> CATTAGCGTCAGACGATAAATTTAGCCGGAACTAAAACACTCTTGTATCATCGCCTTGTAGCG;> ATTAAAGATCGGCACGGAGATATCTTTGACCCCCACTAAAACCGCTTTT;> AAGGGCGACATTCAATAAGTTTACCAGAATGAAATTTTACAG;> TTTTTTTTTTTGGTTTACCAGCGCCACAATAGAAAGCAGA;> TTTTTTTTTTTAGTCAGAAGCAACTCCAACAGGTTTTTTTTTTT;> AAGCGGAGGAGAAGGAACCCTAAATCACCATCAATATGATTTTTTTTTTT;> TTGCATCAAATCAGTAAATATTCATTGACCAGAGGGGGTAATAGTAAAA;> CAAACGTGACTCCTCGCTAATTGAACAAAGTCAGACTCCTCA;> TATTTTGTCACAATAAGACAAGGAACCAGAGCCACCACCGTTTTTTTTTT;> AATTCGAGCTTCAAAGCGAACTCCTTTTCTGTAGCTCAACATGTTTTAA;> TGATAGACGGTTTTTCGCCCTTTGACGTTGGAGTCCACGTTCTTTAATAGTGGACTCTTGTTCCAAACTGGAACAACACTCAACCCTATCTCGGGCTATTCTTTTGATTTATAAGGGATTTTGCCGATTTCGGAACCACCATCAAACAGGATTTTCGCCTGCTGGGGCAAACCAGCGTGGACCGCTTGCTGCAACTCTCTCAGGGCCAGGCGGTGAAGGGCAATCAGCTGTTGCCCGTCTCACTGGTGAAAAGAAAAACCACCCTGGCGCCCAATACGCAAACCGCCTCTCCCCGCGCGTTGGCCGATTCATTAATGCAGCTGGCACGACAGGTTTCCCGACTGGAAAGCGGGCAGTGAGCGCAACGCAATTAATGTGAGTTAGCTCACTCATTAGGCACCCCAGGCTTTACACTTTATGCTTCCGGCTCGTATGTTGTGTGGAATTGTGAGCGGATAACAATTTCACACAGGAAACAGCTATGACCATGATTACGAATTCGAGCTCGGTACCCGGGGATCCTCAACTGTGAGGAGGCTCACGGACGCGAAGAACAGGCACGCGTGCTGGCAGAAACCCCCGGTATGACCGTGAAAACGGCCCGCCGCATTCTGGCCGCAGCACCACAGAGTGCACAGGCGCGCAGTGACACTGCGCTGGATCGTCTGATGCAGGGGGCACCGGCACCGCTGGCTGCAGGTAACCCGGCATCTGATGCCGTTAACGATTTGCTGAACACACCAGTGTAAGGGATGTTTATGACGAGCAAAGAAACCTTTACCCATTACCAGCCGCAGGGCAACAGTGACCCGGCTCATACCGCAACCGCGCCCGGCGGATTGAGTGCGAAAGCGCCTGCAATGACCCCGCTGATGCTGGACACCTCCAGCCGTAAGCTGGTTGCGTGGGATGGCACCACCGACGGTGCTGCCGTTGGCATTCTTGCGGTTGCTGCTGACCAGACCAGCACCACGCTGACGTTCTACAAGTCCGGCACGTTCCGTTATGAGGATGTGCTCTGGCCGGAGGCTGCCAGCGACGAGACGAAAAAACGGACCGCGTTTGCCGGAACGGCAATCAGCATCGTTTAACTTTACCCTTCATCACTAAAGGCCGCCTGTGCGGCTTTTTTTACGGGATTTTTTTATGTCGATGTACACAACCGCCCAACTGCTGGCGGCAAATGAGCAGAAATTTAAGTTTGATCCGCTGTTTCTGCGTCTCTTTTTCCGTGAGAGCTATCCCTTCACCACGGAGAAAGTCTATCTCTCACAAATTCCGGGACTGGTAAACATGGCGCTGTACGTTTCGCCGATTGTTTCCGGTGAGGTTATCCGTTCCCGTGGCGGCTCCACCTCTGAAAGCTTGGCACTGGCCGTCGTTTTACAACGTCGTGACTGGGAAAACCCTGGCGTTACCCAACTTAATCGCCTTGCAGCACATCCCCCTTTCGCCAGCTGGCGTAATAGCGAAGAGGCCCGCACCGATCGCCCTTCCCAACAGTTGCGCAGCCTGAATGGCGAATGGCGCTTTGCCTGGTTTCCGGCACCAGAAGCGGTGCCGGAAAGCTGGCTGGAGTGCGATCTTCCTGAGGCCGATACTGTCGTCGTCCCCTCAAACTGGCAGATGCACGGTTACGATGCGCCCATCTACACCAACGTGACCTATCCCATTACGGTCAATCCGCCGTTTGTTCCCACGGAGAATCCGACGGGTTGTTACTCGCTCACATTTAATGTTGATGAAAGCTGGCTACAGGAAGGCCAGACGCGAATTATTTTTGATGGCGTTCCTATTGGTTAAAAAATGAGCTGATTTAACAAAAATTTAATGCGAATTTTAACAAAATATTAACGTTTACAATTTAAATATTTGCTTATACAATCTTCCTGTTTTTGGGGCTTTTCTGATTATCAACCGGGGTACATATGATTGACATGCTAGTTTTACGATTACCGTTCATCGATTCTCTTGTTTGCTCCAGACTCTCAGGCAATGACCTGATAGCCTTTGTAGATCTCTCAAAAATAGCTACCCTCTCCGGCATTAATTTATCAGCTAGAACGGTTGAATATCATATTGATGGTGATTTGACTGTCTCCGGCCTTTCTCACCCTTTTGAATCTTTACCTACACATTACTCAGGCATTGCATTTAAAATATATGAGGGTTCTAAAAATTTTTATCCTTGCGTTGAAATAAAGGCTTCTCCCGCAAAAGTATTACAGGGTCATAATGTTTTTGGTACAACCGATTTAGCTTTATGCTCTGAGGCTTTATTGCTTAATTTTGCTAATTCTTTGCCTTGCCTGTATGATTTATTGGATGTTAATGCTACTACTATTAGTAGAATTGATGCCACCTTTTCAGCTCGCGCCCCAAATGAAAATATAGCTAAACAGGTTATTGACCATTTGCGAAATGTATCTAATGGTCAAACTAAATCTACTCGTTCGCAGAATTGGGAATCAACTGTTATATGGAATGAAACTTCCAGACACCGTACTTTAGTTGCATATTTAAAACATGTTGAGCTACAGCATTATATTCAGCAATTAAGCTCTAAGCCATCCGCAAAAATGACCTCTTATCAAAAGGAGCAATTAAAGGTACTCTCTAATCCTGACCTGTTGGAGTTTGCTTCCGGTCTGGTTCGCTTTGAAGCTCGAATTAAAACGCGATATTTGAAGTCTTTCGGGCTTCCTCTTAATCTTTTTGATGCAATCCGCTTTGCTTCTGACTATAATAGTCAGGGTAAAGACCTGATTTTTGATTTATGGTCATTCTCGTTTTCTGAACTGTTTAAAGCATTTGAGGGGGATTCAATGAATATTTATGACGATTCCGCAGTATTGGACGCTATCCAGTCTAAACATTTTACTATTACCCCCTCTGGCAAAACTTCTTTTGCAAAAGCCTCTCGCTATTTTGGTTTTTATCGTCGTCTGGTAAACGAGGGTTATGATAGTGTTGCTCTTACTATGCCTCGTAATTCCTTTTGGCGTTATGTATCTGCATTAGTTGAATGTGGTATTCCTAAATCTCAACTGATGAATCTTTCTACCTGTAATAATGTTGTTCCGTTAGTTCGTTTTATTAACGTAGATTTTTCTTCCCAACGTCCTGACTGGTATAATGAGCCAGTTCTTAAAATCGCATAAGGTAATTCACAATGATTAAAGTTGAAATTAAACCATCTCAAGCCCAATTTACTACTCGTTCTGGTGTTTCTCGTCAGGGCAAGCCTTATTCACTGAATGAGCAGCTTTGTTACGTTGATTTGGGTAATGAATATCCGGTTCTTGTCAAGATTACTCTTGATGAAGGTCAGCCAGCCTATGCGCCTGGTCTGTACACCGTTCATCTGTCCTCTTTCAAAGTTGGTCAGTTCGGTTCCCTTATGATTGACCGTCTGCGCCTCGTTCCGGCTAAGTAACATGGAGCAGGTCGCGGATTTCGACACAATTTATCAGGCGATGATACAAATCTCCGTTGTACTTTGTTTCGCGCTTGGTATAATCGCTGGGGGTCAAAGATGAGTGTTTTAGTGTATTCTTTTGCCTCTTTCGTTTTAGGTTGGTGCCTTCGTAGTGGCATTACGTATTTTACCCGTTTAATGGAAACTTCCTCATGAAAAAGTCTTTAGTCCTCAAAGCCTCTGTAGCCGTTGCTACCCTCGTTCCGATGCTGTCTTTCGCTGCTGAGGGTGACGATCCCGCAAAAGCGGCCTTTAACTCCCTGCAAGCCTCAGCGACCGAATATATCGGTTATGCGTGGGCGATGGTTGTTGTCATTGTCGGCGCAACTATCGGTATCAAGCTGTTTAAGAAATTCACCTCGAAAGCAAGCTGATAAACCGATACAATTAAAGGCTCCTTTTGGAGCCTTTTTTTTGGAGATTTTCAACGTGAAAAAATTATTATTCGCAATTCCTTTAGTTGTTCCTTTCTATTCTCACTCCGCTGAAACTGTTGAAAGTTGTTTAGCAAAATCCCATACAGAAAATTCATTTACTAACGTCTGGAAAGACGACAAAACTTTAGATCGTTACGCTAACTATGAGGGCTGTCTGTGGAATGCTACAGGCGTTGTAGTTTGTACTGGTGACGAAACTCAGTGTTACGGTACATGGGTTCCTATTGGGCTTGCTATCCCTGAAAATGAGGGTGGTGGCTCTGAGGGTGGCGGTTCTGAGGGTGGCGGTTCTGAGGGTGGCGGTACTAAACCTCCTGAGTACGGTGATACACCTATTCCGGGCTATACTTATATCAACCCTCTCGACGGCACTTATCCGCCTGGTACTGAGCAAAACCCCGCTAATCCTAATCCTTCTCTTGAGGAGTCTCAGCCTCTTAATACTTTCATGTTTCAGAATAATAGGTTCCGAAATAGGCAGGGGGCATTAACTGTTTATACGGGCACTGTTACTCAAGGCACTGACCCCGTTAAAACTTATTACCAGTACACTCCTGTATCATCAAAAGCCATGTATGACGCTTACTGGAACGGTAAATTCAGAGACTGCGCTTTCCATTCTGGCTTTAATGAGGATTTATTTGTTTGTGAATATCAAGGCCAATCGTCTGACCTGCCTCAACCTCCTGTCAATGCTGGCGGCGGCTCTGGTGGTGGTTCTGGTGGCGGCTCTGAGGGTGGTGGCTCTGAGGGTGGCGGTTCTGAGGGTGGCGGCTCTGAGGGAGGCGGTTCCGGTGGTGGCTCTGGTTCCGGTGATTTTGATTATGAAAAGATGGCAAACGCTAATAAGGGGGCTATGACCGAAAATGCCGATGAAAACGCGCTACAGTCTGACGCTAAAGGCAAACTTGATTCTGTCGCTACTGATTACGGTGCTGCTATCGATGGTTTCATTGGTGACGTTTCCGGCCTTGCTAATGGTAATGGTGCTACTGGTGATTTTGCTGGCTCTAATTCCCAAATGGCTCAAGTCGGTGACGGTGATAATTCACCTTTAATGAATAATTTCCGTCAATATTTACCTTCCCTCCCTCAATCGGTTGAATGTCGCCCTTTTGTCTTTGGCGCTGGTAAACCATATGAATTTTCTATTGATTGTGACAAAATAAACTTATTCCGTGGTGTCTTTGCGTTTCTTTTATATGTTGCCACCTTTATGTATGTATTTTCTACGTTTGCTAACATACTGCGTAATAAGGAGTCTTAATCATGCCAGTTCTTTTGGGTATTCCGTTATTATTGCGTTTCCTCGGTTTCCTTCTGGTAACTTTGTTCGGCTATCTGCTTACTTTTCTTAAAAAGGGCTTCGGTAAGATAGCTATTGCTATTTCATTGTTTCTTGCTCTTATTATTGGGCTTAACTCAATTCTTGTGGGTTATCTCTCTGATATTAGCGCTCAATTACCCTCTGACTTTGTTCAGGGTGTTCAGTTAATTCTCCCGTCTAATGCGCTTCCCTGTTTTTATGTTATTCTCTCTGTAAAGGCTGCTATTTTCATTTTTGACGTTAAACAAAAAATCGTTTCTTATTTGGATTGGGATAAATAATATGGCTGTTTATTTTGTAACTGGCAAATTAGGCTCTGGAAAGACGCTCGTTAGCGTTGGTAAGATTCAGGATAAAATTGTAGCTGGGTGCAAAATAGCAACTAATCTTGATTTAAGGCTTCAAAACCTCCCGCAAGTCGGGAGGTTCGCTAAAACGCCTCGCGTTCTTAGAATACCGGATAAGCCTTCTATATCTGATTTGCTTGCTATTGGGCGCGGTAATGATTCCTACGATGAAAATAAAAACGGCTTGCTTGTTCTCGATGAGTGCGGTACTTGGTTTAATACCCGTTCTTGGAATGATAAGGAAAGACAGCCGATTATTGATTGGTTTCTACATGCTCGTAAATTAGGATGGGATATTATTTTTCTTGTTCAGGACTTATCTATTGTTGATAAACAGGCGCGTTCTGCATTAGCTGAACATGTTGTTTATTGTCGTCGTCTGGACAGAATTACTTTACCTTTTGTCGGTACTTTATATTCTCTTATTACTGGCTCGAAAATGCCTCTGCCTAAATTACATGTTGGCGTTGTTAAATATGGCGATTCTCAATTAAGCCCTACTGTTGAGCGTTGGCTTTATACTGGTAAGAATTTGTATAACGCATATGATACTAAACAGGCTTTTTCTAGTAATTATGATTCCGGTGTTTATTCTTATTTAACGCCTTATTTATCACACGGTCGGTATTTCAAACCATTAAATTTAGGTCAGAAGATGAAATTAACTAAAATATATTTGAAAAAGTTTTCTCGCGTTCTTTGTCTTGCGATTGGATTTGCATCAGCATTTACATATAGTTATATAACCCAACCTAAGCCGGAGGTTAAAAAGGTAGTCTCTCAGACCTATGATTTTGATAAATTCACTATTGACTCTTCTCAGCGTCTTAATCTAAGCTATCGCTATGTTTTCAAGGATTCTAAGGGAAAATTAATTAATAGCGACGATTTACAGAAGCAAGGTTATTCACTCACATATATTGATTTATGTACTGTTTCCATTAAAAAAGGTAATTCAAATGAAATTGTTAAATGTAATTAATTTTGTTTTCTTGATGTTTGTTTCATCATCTTCTTTTGCTCAGGTAATTGAAATGAATAATTCGCCTCTGCGCGATTTTGTAACTTGGTATTCAAAGCAATCAGGCGAATCCGTTATTGTTTCTCCCGATGTAAAAGGTACTGTTACTGTATATTCATCTGACGTTAAACCTGAAAATCTACGCAATTTCTTTATTTCTGTTTTACGTGCAAATAATTTTGATATGGTAGGTTCTAACCCTTCCATTATTCAGAAGTATAATCCAAACAATCAGGATTATATTGATGAATTGCCATCATCTGATAATCAGGAATATGATGATAATTCCGCTCCTTCTGGTGGTTTCTTTGTTCCGCAAAATGATAATGTTACTCAAACTTTTAAAATTAATAACGTTCGGGCAAAGGATTTAATACGAGTTGTCGAATTGTTTGTAAAGTCTAATACTTCTAAATCCTCAAATGTATTATCTATTGACGGCTCTAATCTATTAGTTGTTAGTGCTCCTAAAGATATTTTAGATAACCTTCCTCAATTCCTTTCAACTGTTGATTTGCCAACTGACCAGATATTGATTGAGGGTTTGATATTTGAGGTTCAGCAAGGTGATGCTTTAGATTTTTCATTTGCTGCTGGCTCTCAGCGTGGCACTGTTGCAGGCGGTGTTAATACTGACCGCCTCACCTCTGTTTTATCTTCTGCTGGTGGTTCGTTCGGTATTTTTAATGGCGATGTTTTAGGGCTATCAGTTCGCGCATTAAAGACTAATAGCCATTCAAAAATATTGTCTGTGCCACGTATTCTTACGCTTTCAGGTCAGAAGGGTTCTATCTCTGTTGGCCAGAATGTCCCTTTTATTACTGGTCGTGTGACTGGTGAATCTGCCAATGTAAATAATCCATTTCAGACGATTGAGCGTCAAAATGTAGGTATTTCCATGAGCGTTTTTCCTGTTGCAATGGCTGGCGGTAATATTGTTCTGGATATTACCAGCAAGGCCGATAGTTTGAGTTCTTCTACTCAGGCAAGTGATGTTATTACTAATCAAAGAAGTATTGCTACAACGGTTAATTTGCGTGATGGACAGACTCTTTTACTCGGTGGCCTCACTGATTATAAAAACACTTCTCAGGATTCTGGCGTACCGTTCCTGTCTAAAATCCCTTTAATCGGCCTCCTGTTTAGCTCCCGCTCTGATTCTAACGAGGAAAGCACGTTATACGTGCTCGTCAAAGCAACCATAGTACGCGCCCTGTAGCGGCGCATTAAGCGCGGCGGGTGTGGTGGTTACGCGCAGCGTGACCGCTACACTTGCCAGCGCCCTAGCGCCCGCTCCTTTCGCTTTCTTCCCTTCCTTTCTCGCCACGTTCGCCGGCTTTCCCCGTCAAGCTCTAAATCGGGGGCTCCCTTTAGGGTTCCGATTTAGTGCTTTACGGCACCTCGACCCCAAAAAACTTGATTTGGGTGATGGTTCACGTAGTGGGCCATCGCCC;> TTTTTTTTTTACTAAAGACTTTTTCATACAGAGGGAGCCT;> TTTTTTTTTTACAGACCAGGCGAGCTGCTCATTCTTTTTTTTTT;> CATAGGCTGGCTGATTTGAAAGAGGACAGATGAACGGTGTTTTTTTTTTT;> CCTTCATTTACCCAAACACCAAATTTCACCAGTCAGGACGTTGGGAA;> GGCTTGCGACAACATAAACAAGTCTTTCCAGACGTTAGTAAAGTATGGG;> CTCAGCAGAATTTCAACAACTCAGACAGCCCTCATAGTTAGCTGAGAAT;> AGGGTAGCAACGGCTGAGGAAGTTTCCATTAAACGCGGAACGTTATCAG;> GTTGCGCCGACAATAGGGAGTCAGAGCCCGTTTTCGTGAATTATCACAA;> ACCGATAAGCGGAGGTAACGATCTAAAGTTTTGTCCTTTCAA;> TTAAACAGCTTGATGCGGGATAGCCGCCTCATAGCGACGGAATTAGAGCCAGCA;> TTTTTTTTTTGCTCCAAAAGCTTTGAGGTTTTTTTTTT;> TTTTTTTTTTAGTGAATAAGGCGAATTACCTTATTTTTTTTTTT;> TAATAATTACAACGTTTCAGGGATAGCATACCGCC;> AATCTCCAGTTTCGTAGGAACCCATGTACCTTTTTTTTTT;> ACTTTAATCATTGTTTGCCCTAATTACGCGTTTACGAAGCAA;> TGAATGGGCTTGAGATGGTTTGAACGAGCAGATAC;> CCTGTAGCATTCCAAAAGGAAGGGTCAGAAAGCGCCGAGGAAAAAGACA;> TCACCAGTACAAACTTTTTCATACTGGTCCGTTCCACAAAGT;> TTTTTTTTTTGTAACACTGAAAAAAAAGTTTTTTTTTT;> AGCGCGAAACAAAGTACAATTTTCGGACCAGAAAAATAAATATAAAC;> ACCTGCTCCCAATCATACCGATATATTCGGCAGGAGG;> GAAAAATCTACGTTCAACTTATAATGGATAAGAAATAGTATAAAGCTAAATCGG;> TTTTTTTTTTCCGTACTCAGGAGGTTTAGAGCCCAA;> TTTTTTTTTTGCGATTTTAAGAACTGGCTTAACGGA;> ACCCTCAGAGCCACCACACCCTCTGCCGTCAACATAAAAGAGCA;> TTTTTTTTTTTAGAAAGATGTAAGAGCATTTTTTTTTT;> TTGAGATTTAGGAACAAAAGGGACGAGAAATCAACGTAACAA;> GGGTTTTGCTCAGTATTAGACAATTGAGTTTTATTCAAGAAATCATTTG;> GAGAGGGTTTAACGTTGCGAACTTGCTTTCGAGGTGCGAAAG;> AAGTATAAGCAGCCAGCAATATATTAAAACCAATCAAACAAA;> GCCCGGAAGGAGTGCGTTGAATTAATTGTATCGGT;> AGGCATATCATCAGACAACATTATTACAGGTTTTTTTTTT;> TCTGAAACATGATGTAGTAAAGAACCGGATATTCACAAGAGT;> CTATTATGGCAGGTCAATATCGCGTTTTTTTGCGGATGGCGT;> TCGGAACATTTTGCACCATCGCCCACGCATAACAATTTTTCT;> GCCCCCTTGATATTTGATTAAAGAAAATCAGACGAAGTATCA;> GTGCCCGTCCTCATGAATACCGGCAACAAAAAGGTATTCTTA;> TTTTTTTTTTTTTTGATGATACATAGGTGTATCATTTTTTTTTT;> TTTTTTTTTTACACTATCAACTGGATAGTTTTTTTTTT;> CAGACGACGATAAAATAACGCTACCACATTAATAAAACGAACCATTATA;> AACCAAAATAGCGACAAAAGAAATCTTGAAGGGAACCGAACTGACCAAC;> TAAAGCCCCCTCAGCGTCACCACGAAGGCACCAACGCGATTATACCA;> GAATTTAAATAAGTTTGATATACCCTCAGAACCGCCCCTCAT;> AGTTTTGATCCCCCTGACCATAAATCAAAAAAAGATTAAGAG;> GCATTGATCGCTGAGAGGCGCAGACGGTATGTTACTGTGTCGAAATCCGCG;> GCCGCCATTGGCCTGCCTATTAGAGAAGGATTAGGAACACCCATCAGAG;> GCCACCAAGAATGGTGCCTTGGGATAAGAGAACCGCC;> CCTCAGATTGCCATGAGGGAGGGAAGGTGAAACGCACGCAAT;> TTTTTTTTTTGAACCGCCTCCCGTCATACATGGCTTTTTTTTTT;> TTTTTTTTTTCGTCCAATACTGCGGATGTTTAGTAACCCT;> ATCGTCAGTCTTTACCCTGACTATTATTTTTTTTTT;> GATTAAGAATCATATCGCCATATTTAACAACGCTTTTTTTTTT;> AGGTCATTGCCTGAAGAGGGTAACCAGGCAGCTGGTGGGTAACGCCAGG;> TTTTTTTTTTTACCTGAGCGAAGAGTCATTTTTTTTTT;> TTTTTTTTTTTAATCGTAAAACATTTTGTTAAAATTTTTTTTTT;> TATGTACATTTAAACTCATTTTTTAACCGGCCTTC;> ACATCGGTTTTTTAAGATAAGTTCTGTCACATACA;> CTGATTGTTTGCACGTAAAACTCCCGACAAGCCGTTTAAGCCAATAACG;> TTACAAAGAACCTAAGATGATGGCAATTCCAGAAGTTAAAAGTTTGAGT;> ATCGCGCCAGTTGGCACCTTGAGAAAGCAACAGGAGGCCGAT;> AATTATTTTCTGAAATAATCCTGATTGTTTTTTTTT;> ACTGGCACACAAACCCACCACTAAAGGCGAAAGAGGCAAAAGAATACAC;> CAAAAGACCACAAGGGGAGAATTAACTGATTAGCGAGTTAATCAGTTTC;> AGGAAACAGTCTCTCCGCCACACAGCATGGTAAAATACGTAATGCCACT;> TTTTTTTTTTAAGAAAAGTAAATTCATATTTTTTTTTT;> TTTTTTTTTTCAGGATTAGAGAATATGCAACTAATTTTTTTTTT;> GTACCTTCAATAAAAAGCAATCAAGAGATAGCTGATAAATTA;> CAATAATAAACAGGGAAGCGCACCAGGCAGTAACAAGAAAGG;> TACCGAATCAAAAAATAAGAAACGATTTTTTTTTTTTTTT;> GGTTAGAGCTTAATTGCTGAAAAAAGTATTAAGAGGCTGAGA;> TTTTTTTTTTTGTTTAACGGCCCTTTTTTTTTTTTTTT;> ATTCTGCGAACGCGCGAGCAGCAAATCCCGGTT;> TTTTTTTTTTTACAATTTTATCCTGAATCAATCCAATGAAAAT;> TTTTTTTTTTAGTACGGTGTCTGGAAGTTGACCATTTAGCTAT;> TGCCAGTTACAAAATATTTCCAGAGGTTTTAAAATTACTTTGAAAAAGGAA;> ATATTATTTATCCCTTACCAAAGATTAGAGGGTTA;> AAATCACCAGTAGCACCATTATACAAAAAGTAATCCTGAA;> GCAGCACCGTCAGAAAGAAAGACTTCAAGTATGTTCA;> TTTTTTTTTTTGGTCAATAGGCAAGGCATTTTTTTTTT;> TTTGGGGAGTAGATTTAGTTTTCATTCCATATAACAGTTGATTCCCA;> GTGGCATATAGAAGTGAAAACAGGAAGAACGCCATCA;> TCATACAACCTGTTAGATACATTTCGCAAATTTTTTTTTT;> GCAAATCATGCAGAATACAAAGGCTATCAGAAAAGCCCCAAA;> CATTACCCAACAATATGGAAACCTTGCTAAAAATA;> TTCATCGCGTTTTAGCGAACCAGAAATAAATAACGCTAAAAT;> CATCGAGCTAATTTAATTAATGAATCCTTGAAAAC;> CCAAGTATAAATCACGCTAACGAGCGTCAACAGCCAGAGAAT;> GAACGGGGCTATCTTAGCCGAAGTAAGCTCAGAGCCGCCACCCTCAGAA;> TTTTTTTTTTTTATCATTCCAATTTGCACCCAGCTTTTTTTTTT;> TTTTTTTTTTAAGAATTAGTTCAACGCATTTTTTTTTT;> AATAATATACCGACTATAAAAAAATATTCCCCTTATTAGCGT;> ACGAGCACAGTAATCCACGGAACCGATTCTTTTCATAATCAAAATCACC;> TGACCCTGCAATGCTGAGAAAGGCCGGAATGCCGGGAGTCTG;> AACATTAGAAGCCCACGAGAATCAAATGCTTTAAATTTTTTGGAGGCGA;> AAACAACATGTTAGTCAAGTTTGCCTGTTAATCAGAATGAAACCATCGATA;> CGACAATTGTTTATGCGCCCACGGTATTCTAAGAA;> TATAAAGTCCCATCAACAAGCTTGCGGGAGCCTAATT;> AAGAGAAACGCTCAAACCTCCGGCTTAGTCCCTTATACATTT;> TTTTTTTTTTCAACATGTAATTGGCTGTCTTTCCTTTTTTTTTT;> TTTTTTTTTTAGGATAAAAATTTTTACCTTTATCAAAATT;> GGTACTAGAAAAAGCGTCACCTAGCGACAGCGTCACCGACTTAGCAAGGCCGGAAACCTGTTT;> TTGAGAAGGTCTGAGAGACTAATAGCGACATCAAG;> GACAGTCCATATATTTTAAATGTAATACCAGAGCAGTAGCAT;> ATAAGAAGACCGTGTAGTTAATTTCATCATGGATTCCGAACG;> GCGTTAATATGCGTTACCATTGAGCCATTTGGGAAATTATTCTAAAGGT;> TATATAACTATAAGATCGTCGAATTACCGAGAAAC;> CCTTTTTACAGTAGGGCTTAATTCGAGCTGTAGAA;> TTTTTTTTTTATAGTGAATTTATCAAACGCTGAAAAAGAA;> TTTTTTTTTTATTCAACCGTTCATCGATGAACGGTTTTTTTTTT;> AGCTATTAAAAGGGCTGAGTAATGTGTAGCCCAAATTGTATAAGATCAA;> TTTGAGAGATCTATAGCAGAAGCCAATCGTCTGAATTCTGACCTAAA;> CTATTAATAGCCCTAGTCACACTGTCCATTGCCTGAGTAG;> TAGCTTACAATATTGATAGAAAGAAGTGTTTTTATGGAGCTAGAAAGGA;> GACGGGGATCGGCAAATCCTGTTTGATGGTTTTTTTTTTT;> ATCAAACGGTGAAGAACGTCAAGAATGCCAACGGCGCGCTTT;> ACAGCGGGGGAACACGTAACCTCAATCAGAGCAAAAAAGCCTTTTTGCG;> AAGAACGTGGACTCTTGAGGATTAGAGCTATACAGTAAATCAACGCGCC;> GGGTTGAGTGTTGTCTCGTATAGGTTATGATTCGCAACAATT;> AAATCCCTTATAAACCGATTTACATACGAGCTGTTTCCTGTG;> TTTTTTTTTTGGTTCCGAAAAAGCCGGCTTTTTTTTTT;> AAATCCCGTAAATCCGTTTTTTCGTCCTCATAATATCAGG;> TTTTTTTTTTCTTTTCACCAGTGAGACGGAGGCGAA;> TTTTTTTTTTTCATTTGCCGCCAGCAGTTCGGCCTTTTGCCGTTCCGGCA;> CGTTAATTAGCATGGTGCATCCTCAGGACCGGAAT;> TTGTAAAATTTTCATAACATCTAATTGCCAGACCG;> GGTTTAACGTCAGAGCTTATCATAGCAAAATTGAGTATTACGCAGACGA;> ATTTTCAACCTTTTTAACAACTATTAACCCACACCACTATGG;> AAGAAATTGCGTAGCGCGAGGTAGGAATAGATAAC;> TTTTTTTTTTGGATTATACCATTTCAATTTTTTTTTTT;> AAAATAATTCGCGTCTAATAGGATTGTATATGAAAAGTTCTACTGGTCATT;> TTTTTTTTTTTTGCGGAACAAAGAAACCACATCAATTAATGGATTGCTAT;> TTTTTTTTTTTTCGCATTAAATTTTTGTTCATCAACTCTCCGT;> TTCCTGATTATCCCATATCGAAGCCTCCGCACTAGAAACA;> AGACAAAGATAATAAAAATGCGCCCAGCAGTTGAGGA;> TTTAATGGTTTGAAATACCTAAACACTGAATAACAGTACATAACAGT;> TTTTTTTTTTTAACAACCCTTGAGGGGATTTTTTTTTT;> GATTGACCGAGAGACGCAGAATGTGTACATCGACATAAAA;> CGTAATGGGATAATAATACATCAACGTCCCCACTAGGCCAGA;> TAAATCCTTTGCCCCGAGATATCGGAACAGTGTAA;> TGCCAGTGTCGGATATTAAATGTGAGCGAGTTTTTTTTTT;> GTAGATGCCAGCTTACAGCGCCGCCACGCGGGGTC;> CGTCAATAAACAGACGGAAACAATCGGCGCGATGGAAAGGGCGAAAAAC;> ATCTGGTAGAGGCGGATGATGAATAATCTAGGCAGAGGCATT;> TTTTTTTTTTCCCTCAATCAATAACATTATCATTTTTTTTTTTT;> TTTTTTTTTTCGACGACAGCAACTGTTGTTTTTTTTTT;> ACTCCAGGGCGCATAACGGCGCTGTAGCCAGCTTTAAATCAG;> GGTGAGGAACCACCATGTGAGCGGAATCATAATTAAAGATTC;> CGGTCAGTAATAGATTTAGAAGTATTAGACTATTACAAATCATAATTGC;> TGCCACGCGGTCACACGTATATTTCACGGTTAACGGCATCAGATGCCGG;> CTGAGAGGAACTGATTAATTTGTTGGGTCCAGTATAAAGCCA;> CAAATGACTAGGGCTTAGAATGGCCAGAGTTACCTGCAGCCAGCGGTGC;> AAAACATGCAACAGATCTTTAAAACAATTCGACAATCCAGTT;> TTTGAATAAAGCATCAAATCAATTAATTGAGCGGAATTATCATCATA;> TTTTTTTTTTTAAGAATACGTGTCAAATATCAAATTTTTTTTTT;> TTTTTTTTTTGGAAGGGCGATCGGTGGGCTGCGTATCGGC;> CGGGCCTCAGTCACGACGTTGTAAAATTTTTTTTTT;> ATTTACACGTTGTAGCAATTAGGCGCGTCGCCGCGCATCACC;> TTGGCAGTATATTTTGATAAATATGTAAATGCTGAAAAACTTTTTCAAAATTCACC;> GAGGCCACCGAGTATTCCTCGGCTGGCACACTAAA;> AATCCTGCCCTTCTGACCTGAAAGCGTTTTTTTTTT;> TTTTTTTTTTAGGAACGGTACGCCAGTAAAGGGGAGAAAG;> TTTTTTTTTTCGACGGCCAGTGTTGTGAGAGATATTTTTTTTTT;> CCAAGCTCGCACTCGTCACTGTTGCCCTGCGGCTGATTGCAG;> TTCAGAGGTTTTCCCTTCGCTATTACGCCAAAGCG;> GTGGAGCCATGTTTTCTCACGGAAAATCCGGAACGTCGGTGGTGCCATC;> GCTACAGCATTTTGACGCTTGCGCTCATCCGCCAGCCATTGCAA;> GACGAGCGCTGCGCTGGGGTCTGGAACAAGAGTCCACTTTACGGAGCAC;> ACGTGCTAAAGAGTCGACCAGACGCGAGTGCAAATCCAATCGCA;> GAAACGTTCCGGCACCGCTTAAGGGTCACGTTGGTGATAATC;> TTTTTTTTTTGAACGTGGCATTTTAGACTTTTTTTTTT;> TTTTTTTTTTGACTTTCTCCGTTTAAATTTCTGCTTTTTTTTTT;> AGTTTTTGTAACCAACCGCCTCGCCATTTCTGTAA;> GAGGTGCAATGAGTAGGATCCCCGGGTAGGGCCGT;> CCTAAAGGCGGGCGAAAATCTGGCTATTAGTCTTTAGGGACA;> GGAGCCCTCAAAAGTGGTTTGCCCCAGCGCAACAGGCGTATTGGGCGCC;> GAGTTGCAGCAAGCGGCCGCCTGACGCGCGGGGAGAGAGCATAA;> TCCACGCAATAGCCGAACGTTACAGTTGTACCAAGAAAACAA;> GTAATATCCAGAACTCCCTTAAGCACGCGTGCCCG;> AAGAACTCAAACTATCGGCGCAAATCGTCATACACAGTTGGAGCTAA;> CAGGAAAAACAAGGCGATAACCTCACCGCCGCTGGAG;> TTTTTTTTTTAGTTAAACGGCTGGTCTGTTTTTTTTTT;> TCGTCGCTGGCAGCCTGCCCGCTTTCCAGTCGGGAAACCTGTCTCACAT;> CGTGCCAGCTGCATTAATGAAGGTGCCTCGTAAAGAGTGTAG;> GCGTGGTATGCTGATAGTGATGAAGGGTAATTTTTTTTTT;> CTTGTAGGGATAGCACCAGTCAGATCGCCCATTCGCCATTCA;> CCACACAAGAGCTTGAAGGGACTGAACCGCACAGA;> TTTTTTTTTTCCGCTCACAATTAGGGTGGTTTTTTTTTTTTTTT;> TTTTTTTTTTGTCAGCAGCCGGGCGCGGTTTTTTTTTT;> AGCACCGTGCCGGAAACGCGGAAAAGCCGCACAGGGGGCGGT;> ACCAGCTTATGTTCTTCGCGTGTTGCGCTCACTCCCGTGAACCTTAATG;> CCGTGAGCCTCCTCCGGGGGTTTGCTTTAATTAAC;> CGAATTCGTAATCAGTGCTGCCAGAGCGAATCAGTTTCTGGCCAACAGA;> GCATCAGGGAACGGATTAAGTCGAAAGGGGGATGTGATCTGGTGCCGGA;> TTCTGCCCACTGGTGTGTTCACTTGCTGAGTAATAACATCACTCACGCA;> ATGCGGCCCGAGCTAGCCTGGTCGGCCAGCCCTGAGA;> CTCTGTGTGGTCATAGCCGGAGCGGTTTCTGATTGCCCTTCA;> TGCGCGCCTGTGCACGGTGCCCCCTGCATCAGACGATCCATTTTTTTTTT;> TTTTTTTTTTGCGCAGTGTCACTGAAATTGTTATTTTTTTTTTT;> TTTTTTTTTTTTGCGGTATGAGCCGGAATCCGCAACCGCA;> GTAATGGGTAAAGGTTTCTTTGTGTCCACCACGCAGCACATC;> GCTCGTCATAAACAAATATTAGGAAATACCACTTCTTTGATT

Here, we addressed the problem of accurate structural validation with cryo-EM-based methodologies for determining the structures of up to megadalton-scale DNA objects in solution, together with molecular-dynamics-based methods for building pseudoatomic models in a semiautomated fashion. The library of objects includes four brick-like multilayer DNA origami objects with increasing internal floppiness, a barrel-like 126-helix bundle, two variants of a multidomain object called Twisttower, a design variant v2 of a previously reported object called the Pointer, a small 16-helix bundle, four variants of a hinged-beam-like object, two variants of a dumbbell-like object, and five variants of a six-helix tube featuring asymmetric markers at either end as reporters for twist and one ten-helix tube. We constructed pseudoatomic models for six different objects. The fitting was validated using Fourier shell correlation against the cryo-EM half-maps and the models show good cross-correlation with the cryo-EM maps.

Since we just saw that crossovers are necessary to transmit the torques, we wondered whether strains originating from crossovers constitute the root cause of twist in honeycomb objects. If this were true, making crossovers floppier should reduce twist deformations. To test this hypothesis, we designed and analyzed a set of multilayer DNA origami 48-helix-brick variants in which we added unpaired thymidines at all staple-strand crossovers (0T, 1T, 2T, and 4T). All variants displayed right-handed global twist deformations of comparable extent, which suggests that strains produced at crossovers do not cause the twist. Since helical details could be discerned in the majority of the helices of the map obtained with the 0T variant, we could determine the handedness of the global twist deformation based on the fact that B-DNA is right-handed. Whereas the global twist remained unaffected, adding the thymidines made the objects swell. The interhelical spacing and the effective diameter of helices increased with T addition, which we attribute to the increasing fluctuations enabled by the increasingly floppy interhelical junctions. To show the efficacy of the multibody refinement even when the object does not have clear domains, we applied the multibody approach to three brick-like objects and the 126-helix bundle. Simply dividing the whole object into smaller rigid bodies (right) enabled reconstructing all regions of the objects in greater detail including the peripheries (top vs. bottom).>[4x]VKVDLESKRYGEKLKEVFLMLDNNVVECIKEITESSRNGKLVFFVGAGVSTLSDYPQWWRLVDKYHEELYGSPKKGNYSSDEYLRIPQIFYNVKGEMAFDGILKDFFQVDKPTNPIHDKILAMNPAHVITTNYDNLIDTACWKRGKYFSVISAEEDVANATSSRYLLKVHGDFRKGFKGENVVLKEDDYLNYDQNYPLISNLMKTIIATHTIVFIGYGLGDYNINMLLNWVRKLQKDSFHKPFFIRTDPSPIENETLIYYENKGLRIIDAASLIDSNEYDYLER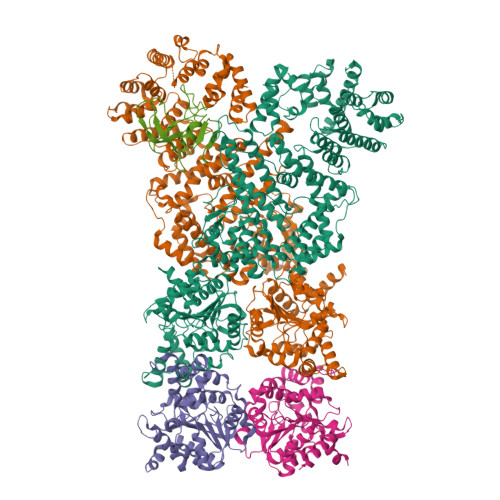YSAVMDLLIESQENKFITKDDEVIDYIYGKISPLFALQYIRKIDLKHVFEYDYHFEVNGTVVRHKNKGFGYMERFFELKESCDERSKLSKKQYERFNALFNFFEKNGVICMAKDAGTLNTSIEINSLAYHGKYDVMKKFIEEQSVSIEDDYKKAFFLACLGRWEESYDLYSNIILNSIDESNGCVYYLSQINRYRIYQSITQAVTQFNGLGLLTFGRHYKPFTDEFLARIEREMTNFNIDDLFNGMPFEFQKKYKILEFLSDNQFLYDDTVKLFELTNKVRSEMSEGSYSFGMSSDIVVLLRLYDNLRFLYENCLWSVSFHEFHQYIRNSMSLLIEKAEYERTRDIDELGFSFFGKKSGFFMEYYDFVNISRHFKIDDIKNLERSCSIDKIRFGEQEKIEEYLVGIAEEITKQFSANGMNVVFYTQFISEAKAALYFAKYVKLSEEGLGKIVKALLFYFPERDLDIGKRYVWLERLTKCNELPKSIISIIDDFLVLQAEKHIDQNYSEVSSNGLYSRDYGALIKHFEKNFISKRLSEITLCLTQDKQKQIDFLFKLLPLLSTNAKSHLLSFKSVENINDLMNGIRIGLIDEFTPEHEELIIEYLETRKVNYIVEKEKGIQTFSSNDYMSTFGIWYFLEEINNSKMEEFIGMDDQYDFFVDPENFDYKKFIPSWLKNYNDKLLGKIAGNKHMKHHVIEVLKERVKNSNDKRYLEILMNYFI;> MIEIFKDTGATHDLVYHSKINTFVWDVEFDIVLSDSKELNKCYFVKCFNPYRINGKCDFAVSSIDIFSEGKRLLIENEFNFKITKAVHVATSKDVTEIVLHLSERISSPFPIVKEVVYLD Non-ribosomal peptide synthetases (NRPS) are multi-modular/domain enzymes that catalyze the synthesis of bioactive peptides. A crucial step in the process is peptide elongation accomplished by the condensation (C) domain with the aid of a peptidyl carrier or thiolation (T) domain. Here, we examined condensation reaction carried out by NRPS AmbB involved in biosynthesis of l-2-amino-4-methoxy-trans-3-butenoic acid (AMB) in P. aeruginosa. We determined crystal structures of the truncated T–C bidomain of AmbB in three forms, the apo enzyme with disordered T domain, the holo form with serine linked phosphopantetheine (Ppant) and a holo form with substrate (l-alanine) loaded onto Ppant.

To obtain AmbB T–C with l-Ala, apo full-length AmbB, which activates l-Ala, was used to trans-aminoacylate l-Ala onto the Ppant of the T domain of AmbB T–C. MS analysis showed a mass shift (+71.04) of the alkylated Ppant arm as compared to holo AmbB T–C, which corresponds to the molecular weight of l-Ala. In the structure of holo AmbB T–C tethered with Ppant-l-Ala, chains B and D exhibit relatively well-defined electron density for Ppant-l-Ala while chains A and C show fragmented density for Ppant-l-Ala. The interactions of Ppant moiety with C domain are essentially identical to those observed in the structure of holo AmbB T–C tethered with Ppant. The thiol moiety of Ppant is covalently attached to the carboxyl group of l-Ala via a thioester bond. The positioning of the Ppant places l-Ala in close vicinity to the active site, with the reactive carbonyl group facing the donor side of the C domain. l-Ala is surrounded by two residues namely Phe1181 and Leu846. In holo AmbB T–C with l-Ala (chain B), the side chain of l-Ala is oriented towards the hydrophobic residues Leu846 and Phe1181 while the free amino group is in close proximity to His953, poised for condensation reaction. Ppant-l-Ala of AmbB follows the same trajectory in the donor side as Ppant-fVal, placing the substrate l-Ala and fVal, at similar distances to the catalytic His953 and His908, respectively. Superimposition of holo AmbB T-C with L-Ala and the T-C bidomain of LgrA, gave an RMSD value of 2.60 Å for 345 Cα, suggesting that AmbB T-C and T-C bidomain of LgrA adopt similar conformations. In addition, the delivery of the substrate l-Ala, did not cause any discernible conformation change in the C domain.

>[4x]TGAEPQALPSDPLEQALHQAWQAQLGAPPRAGQGFYAAGGDSLRAVHLLATLRQRLSRRVPLQAFAGGPATPEALLELLRQAAPEGDEPEPSAGAAGLSLAERRLWVAQQLAPEDTSYNLLAHLRIVGATADAIEQALRQLLERHVALRRRVETGVDGPQPHALAAHAVPLQRLLASDAVHAERLLEDGVRREGARVFDLAHEAPARLLLVVTRDSARADLLLSVHHYAFDDVSLAVFAAELKTLLDGGRLGVLASTPEQVAARERAALASGRLDRVAERWAERLLPLAKAPGAAPARPEESGGRAGQRLALPVSAAVHAACRALAERTSVSPFSAALQAFAEVLGAELGVDDLLVGVALAGRSRLEMQGLVGCFVNLLPLAVGLRPEQSVEWRLRQVGHDLLELLEHQDVPLECVTQALRQRGASGLPIRIACGAHNGRAAPAVDAGVRVEADFIPVPGARLDLTLWLEDQPQGWLAVWTGVSAIFDLHRIERLHQAWERRLLANAGEPISKRMSPEGCNAS>[2x]AGHMTDYVFKAGRKDLAPLLLLHSTGGDEHQLVEIAEMIAPSHPIL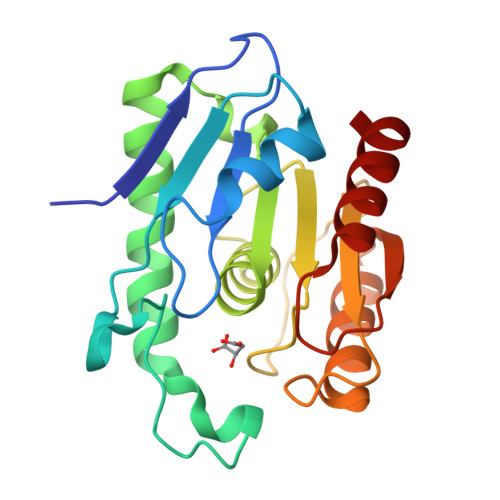SIRGRINEQGVNRYFKLRGLGGFTKENFDLESLDEETDWLTDEVSLLAEKHDLDVHKMIAIGYSNGANVALNMFLRGKINFDKIIAFHGMQLEDFEQTVQLDDKHVFLSYAPNDMIVPQKNFGDLKGDLEDSGCQLEIYESSLGHQLTQEEVLAAKKWLTETK> MASKTIKIMPVGDSCTEGMGGGEMGSYRTELYRLLTQAGLSIDFVGSQRS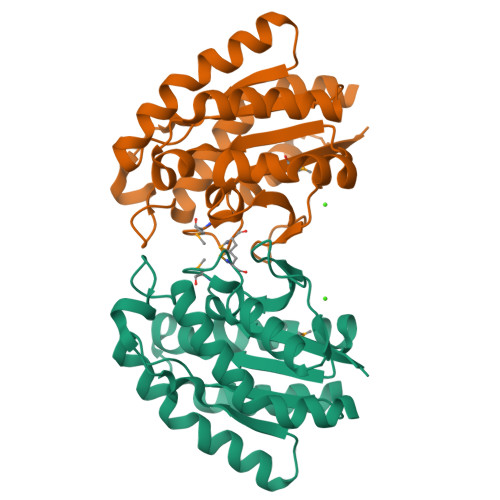GPSSLPDKDHEGHSGWTIPQIASNINNWLNTHNPDVVFLWIGGNDLLLNGNLNATGLSNLIDQIFTVKPNVTLFVADYYPWPEAIKQYNAVIPGIVQQKANAGKKVYFVKLSEIQFDRNTDISWDGLHLSEIGYKKIANIWYKYTIDILRALAGETQLEHHHHHH> MSVLYPLIQALVLFAVAPLLSGITRVARARLHNRRGPGVLQEYRDIIKLLGRQSVGPDASGWVFRLTPYVMVGVMLTIATALPVVTVGSPLPQLGDLITLLYLFAIARFFFAISGLDTGSPFTAIGASREAMLGVLVEPMLLLGLWVAAQVAGSTNISNITDTVYHWPLSQSIPLVLALCACAFATFIEMGKLPFDLAEAEQELQEGPLSEYSGSGFGVMKWGISLKQLVVLQMFVGVFIPWGQMETFT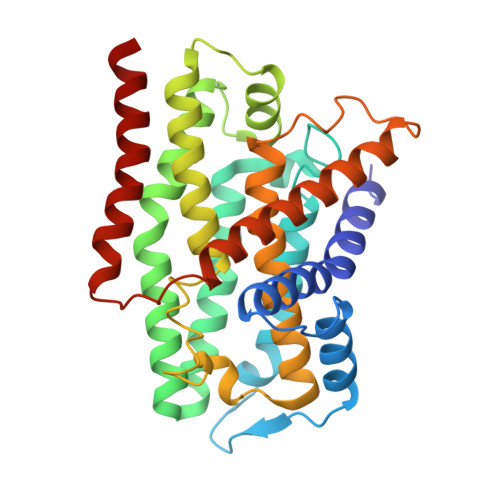AGGLLLALVIAIVKLVVGVLVIALFENSMARLRLDITPRITWAGFGFAFLAFVSLLAA>PLVCLADFKAHAQKQLSKTSWDFIEGEADDGITYSENIAAFKR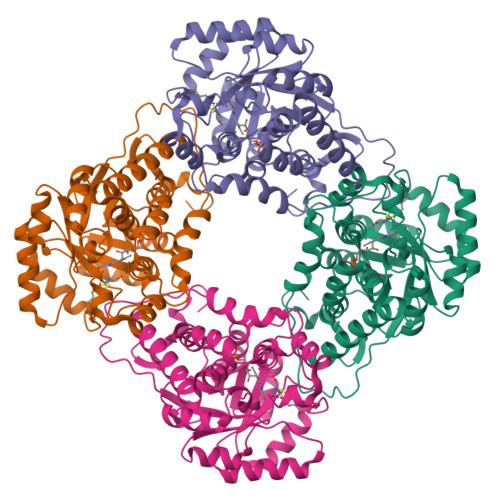IRLRPRYLRDMSKVDTRTTIQGQEISAPICISPTAFHSIAWPDGEKSTARAAQEANICYVISSYASYSLEDIVAAAPEGFRWFQLYMKSDWDFNKQMVQRAEALGFKALVITIDTPVLGNRRRDKRNQLNLEANILKAALRALKEEKPTQSVPVLFPKASFCWNDLSLLQSITRLPIILKGILTKEDAELAMKHNVQGIVVSNHGGRQLDEVSASIDALREVVAAVKGKIEVYMDGGVRTGTDVLKALALGARCIFLGRPILWGLACKGEDGVKEVLDILTAELHRCMTLSGCQSVAEISPDLIQFSRL[3x]> NNFNYGAYHSLEAIYHEMDNIAADFPDLARRVKIGHSFENRPMYVLKFSTGKGVRRPAVWLNAGIHSREWISQATAIWTARKIVSDYQRDPAITSILEKMDIFLLPVA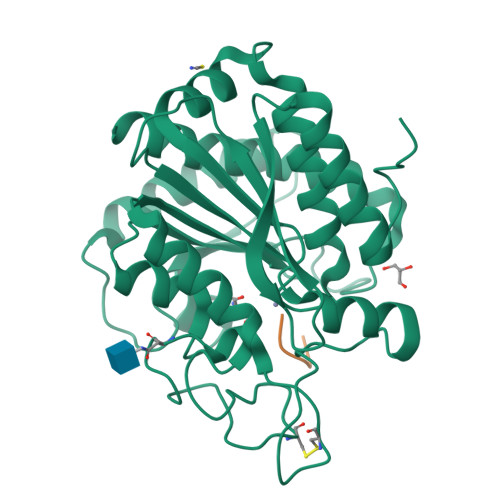NPDGYVYTQTQNRLWRKTRSRNPGSSCIGADPNRNWNASFAGKGASDNPCSEVYHGPHANSEVEVKSVVDFIQKHGNFKGFIDLHSYSQLLMYPYGYSVKKAPDAEELDKVARLAAKALASVSGTEYQVGPTCTTVYPASGSSIDWAYDNGIKFAFTFELRDTGTYGFLLPANQIIPTAEETWLGLKTIMEHVRDNL;> FNRPV>RKIKLEGLSDVASISTKLQNTLIQYHSIKEDEWRVAKKVKDVTVWRKPSEEFNGYLYKAQGVMDDVVNNVIDHIRPGPWRLDWDRLMTSLDVLEHFEENCCVMRYTTAGQLDNIISPREFVDFSYTVGYEEGLLSCGVSVEWSETRPEFVRGYNHPCG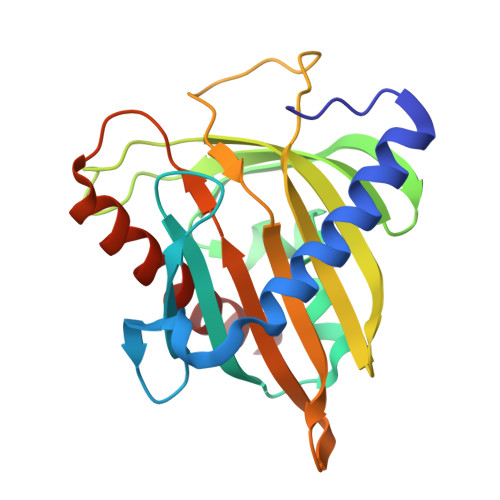WFCVPLKDSPSQSLLTGYIQTDLRGMIPQSAVDTAMASTLANFYSDLRKGLR[2x]>[5x]VSPPPPIADEPLTVNTGIYLIESYSLDDKAETFKVNAFLSLSWKDRRLAFDPVRSGVRVKTYEPEAIWIPEIRFVNVENARDADVVDISVSPDGTVQYLERFSARVLSPLDFRRYPFDSQTLHIYLIVRSVDTRNIVLAVDLEKVGKNDD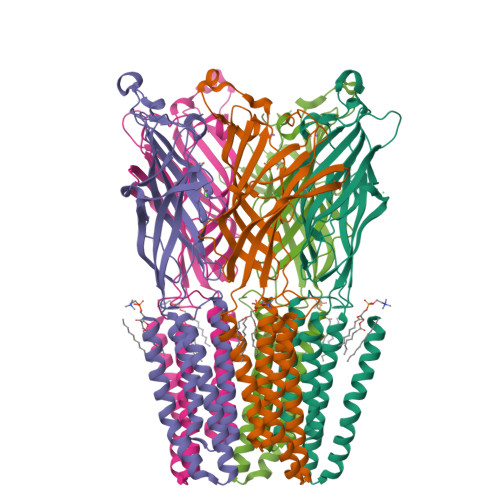VFLTGWDIESFTAVVKPANFALEDRLESKLDYQLRISRCYFSYIPNIILPMLFILFISWTAFWSTSYEANVTLVVSTLIAHIAFNILVETNLPKTPYMTYTGAIIFMIYLFYFVAVIEVTVQHYLKVESQPARAASITRASRIAFPVVFLLANIILAFLFF> MLPRLICINDYEQHAKSVLPKSIYDYYRSGANDEETLADNIAAFSRWKLYPRMLRNVAETDLSTSVLGQRVSMPICVGATAMQRMAHVDGELATVRACQSLGTGMMLSSWATSSIEEVAEAGPEALRWLQLYIYKDREVTKKLVRQAEKMGYKAIFVTVDTPYLGNRLDDVRNRFKLPPQLRMKNFETSTLSFSPEENFGDDSGLAAYVAKAIDPSISWEDIKWLRRLTSLPIVAKGILRGDDAREAVKHGLNGILVSNHGARQLDGVPATIDVLPEIVEAVEGKVEVFLDGGVRKGTDVLKALALGAKA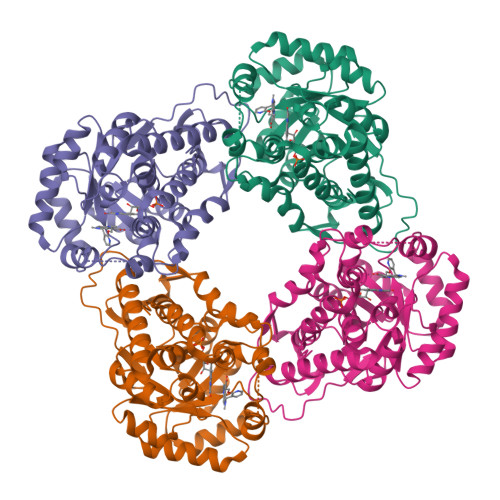VFVGRPIVWGLAFQGEKGVQDVLEILKEEFRLAMALSGCQNVKVIDKTLVRKNPLAVS>[6x]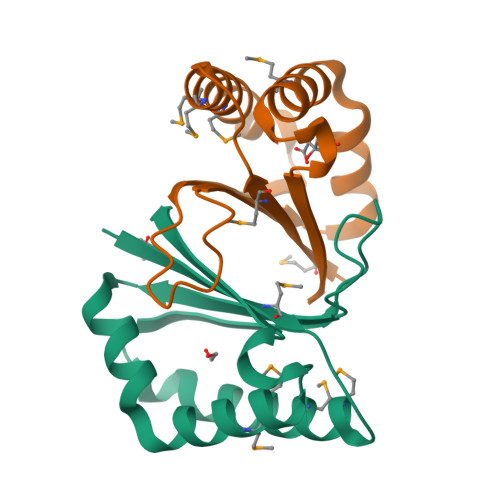MGSDKIHHHHHHENLYFQGMLYHLVMLEPEGEGAMDRIMEAMAILDGLAPELPGLTEFRHGPNRDFEQKSERYPYGFLCTFTDKAALDAYAVHPTHQRAGGMLVASCRNGADGILVVDLEV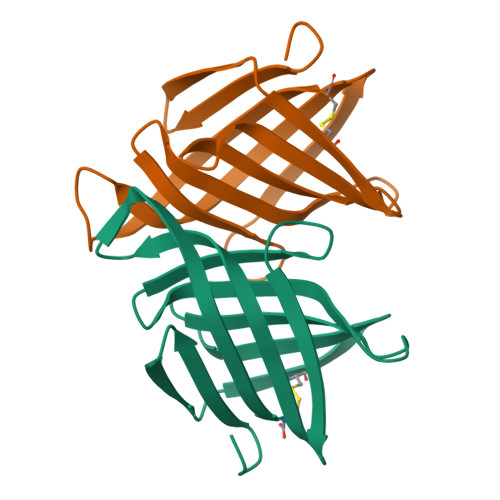>[2x]MAHHHHHHSRPPAQLSSTASVTVDGKDRNFHIVTCRQLEWRRMIDIGADFSGAKVAVDENAQPPVVESVHIQNLSGFSGMYSRGGSGSADMSMTGDKFTISGTADGYKTDKPGEPATATFKIVVTC> GHMTDEDSEANALADPDNPPLSAEQLASAPRMPRIKIIRRALKLTQEEFSARYHIPLGTLR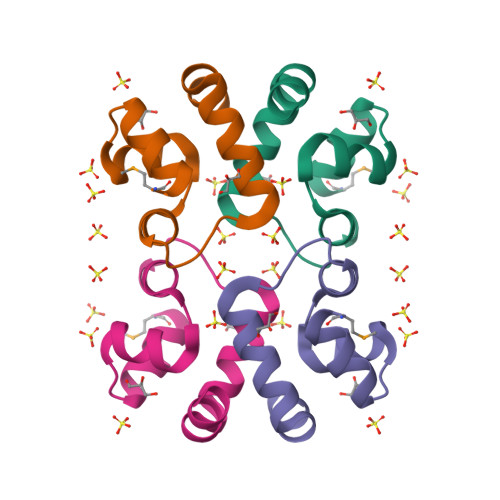DWEQGRSEPDQPARAYLKIIAVDPEGTAAALRKGATGS>MSSKPKPIEIIGAPFSKGQPRGGVEKGPAALRKAGLVEKLKETEYNVRDHGDLAFVDVPNDSPFQIVKNPRSVGKANEQLAAVVAETQKNGTISVVLGGDHSMAIGSISGHARVHPDLCVIWVDAHTDINTPLTTSSGNLHGQPVAFLLKELKGKFPDVPGFSWVTPCISAKDIVYIGLRDVDPGEHYIIKTLGIKYFSMTEVDKLGIGKVMEETFSYLLGRKKRPIHLSFDVDGLDPVFTPATGTPVVGGLSYREGLYITEEIYKTGLLSG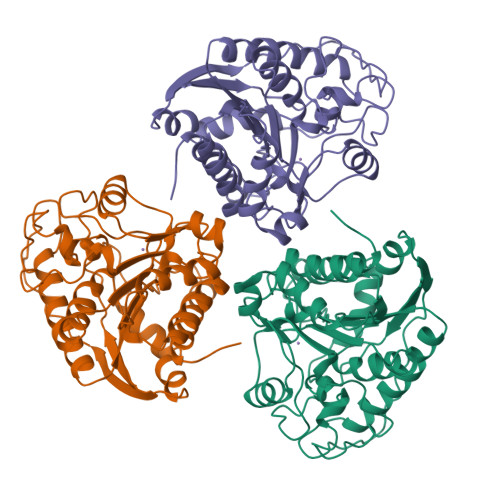LDIMEVNPTLGKTPEEVTRTVNTAVPLTLSCFGTKREGNHKPETDYLKPPK[3x]>[2x]MDSYVEVKGVVGHPV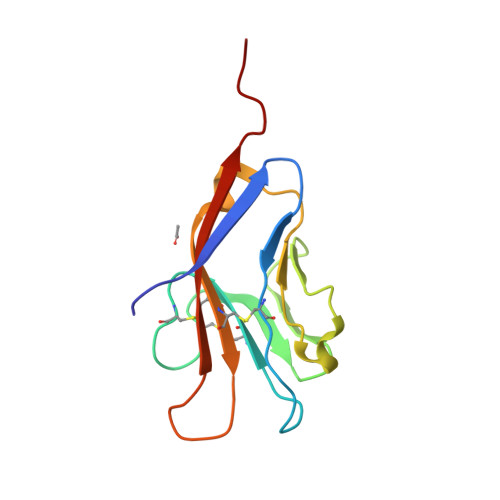TLPCTYSTYRGITTTCWGRGQCPSSACQNTLIWTNGHRVTYQKSSRYNLKGHISEGDVSLTIENSVESDSGLYCCRVEIPGWFNDQKVTFSLQVKPELVPR> DYKDDDDAMGAAISTSIPVISQPQFTAMNEPQCFYNESIAFFYNRSGKHLATEWNTVSKLVMGLGITVCIFIMLANLLVMVAIYVNRRFHFPIYYLMANLAAADFFAGLAYFYLMFNTGPNTRRLTVSTWLLRQGLIDTSLTASVANLLAIAIERHITVFRMQLHTRMSNRRVVVVIVVIWTMAIVMGAIPSVGWNCICDIENCSNMAPLYSDSYLVFWAI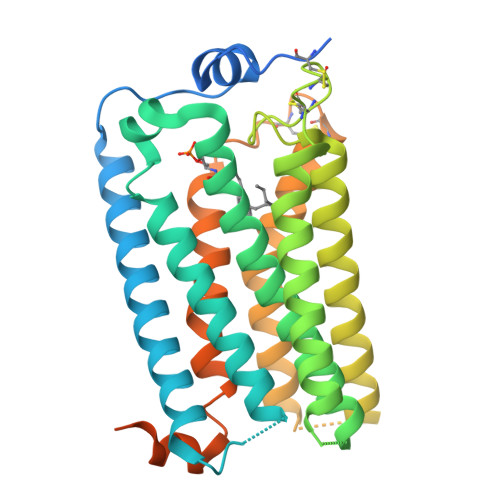FNLVTFVVMVVLYAHIFGYVRQRTMRMSRHSSGPRRNRDTMMSLLKTVVIVLGAFIICWTPGLVLLLLDVCCPQCDVLAYEKFFLLLAEFNSAMNPIIYSYRDKEMSATFRQILCCQRSENPTGPTEGSDRSASSLNHTILAGVHSNDHSVVENLYFQ> MFSLNPQSNGNSNNLFGNVTLGNFSNNSNNLFGGSSTTSTNTNNSNNLFGGSSTTNSNNLFGSGGSSTTNNNNFNSNFNNNNIKNENKIKNGKKFYNFRWSPTGEILLYNTLNNFDNHNFDQKNGGSDTIRYEMNTTLSTIKKFYNDLYTNFETMQRIAGLSNQVIPDDRVREISHHSRTYLSVILAAINQMSKSQKTGSYIDDEDSCMNCDPLDNDLIKIQTPRVLEYFKQYPNKTLIFFCGSIDSIYPYLCSKLSMETKSKCILIARESNVPNSKRLDLIRTISNQGELKILNKDEYSNRYQIANENYGELDDVLTLEIDDTYLAYEREIDNLICMSTMWRVANLFYFSVSSSSNSVSPTQLLDCIELERKELLNSIEQQGTQDPMDSEYYNQIARLLVCGCIDQVIQQLNILSRAPRSASQIKSTSRKSPINLLIDILSSIPLKKKSINGGGGAPLYPNEHLIQWNKWHQETQKILSQYIESGSSSTNQVDENLLPIVKILLGDQQTIMSTCNSFLQLVVSNILFVEYTTSTTQLRQLFT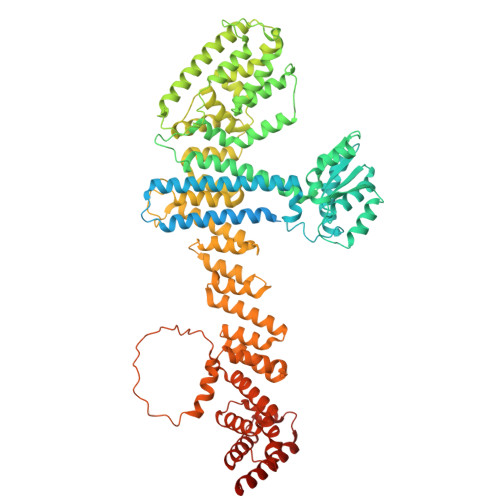QCYQTIQAPTTVDKIFLSFATKDLDITLKKIFKHSPAWLAVHLSDLLYHHPYVMRKLPNSESQLTNIREYLLSDFGQSLASDSSLLSIGCNYLKYVKNGGLEMIDQFISRQPIHFEKNAIKMLDKWATSVETKNSIYKMLSLQDFKRKRYAASLNWLMLANDNSHITLLSNYLLENQLNSEFLNDLQSLLEKNDEIDCNINNNNNNNNNNNSNNRISGNNNNNMIIDENKFEITNNSELIFLIRYRELISLWKERSFKEYSSSLCLMFKDRVIPKRFWLRLLIDCVPLLESLKNLYFTYQDTLLLQSCLEEIIQSHLFDQYSFNISNQDIQILRSALARNLAKSIIS> MRTYSSLLEEFATELGLEEIETNELGHGAVTIDKIWVVHLAPINEKELVAFMRAGILTGQSQLYDILRKNLFSPLSGVIRCALDKDDHWLLWSQLNINDTSGTQLASV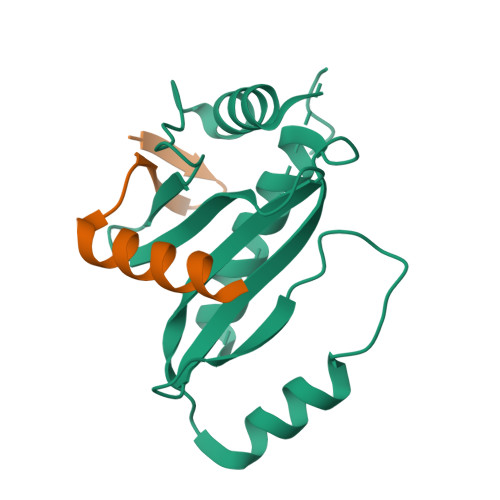LTSLVDKAVTLSCEPTMKKEEDDHRPSSSHLLV;> GDCTGKLRGNVAANKETTFQGLTIASGARESEKVFAQTVLSHV> MSKDFIINEQIRAREVRLIDQNGDQLGIKSKQEALEIAARRNLDLVLVAPNAKPP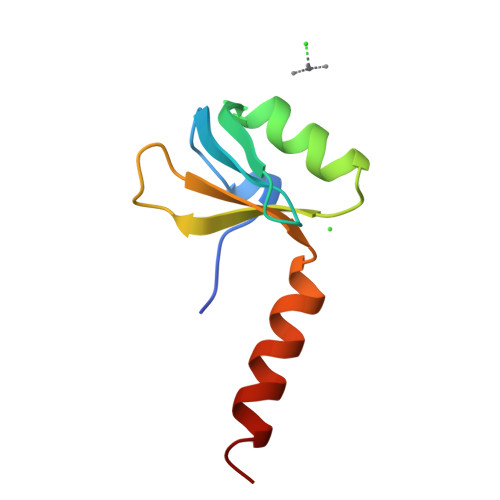VCRIMDYGKFRFEQQKKEKEARK N-(5-{(1S)-1-[(5-fluoro-1,3-benzoxazol-2-yl)amino]ethyl}-2-methylphenyl)imidazo[1,2-a]pyridine-3-carboxamide | C24 H20 F N5 O2 | 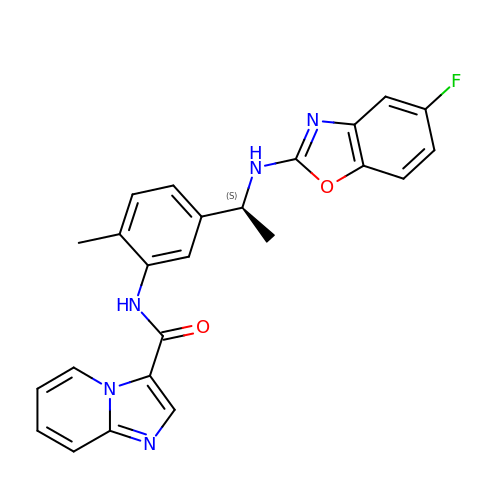YLTBELFOTTYXRF-HNNXBMFYSA-N>MAGMKTASGDYIDSSWELRVFVGEEDPEAESVTLRVTGESHIGGVLLKIVEQINRKQDWSDHAIWWEQKRQWLLQTHWTLDKYGILADARLFFGPQHRPVILRLPNRRALRLRASFSQPLFQAVAAICRLLSIRHPEELSLLRAPEKKEKKKKEKEPEEELYDLSYHMLSRPQPPPDPLLLQRLPRPSSLSDKTQLHSRWLDSSRCLMQQGIKAGDALWLRFKYYSFFDLDPKTDPVRLTQLYEQARWDLLLEEIDCTEEEMMVFAALQYHINKLSQSGEVGEPAEGLNPYGLVAPRFQRKFKAKQLTPRILEAHQNVAQLSLAEAQLRFIQAWQSLPDFGISYVMVRFKGSRKDEILGIANNRLIRIDLAVGDVVKTWRFSNMR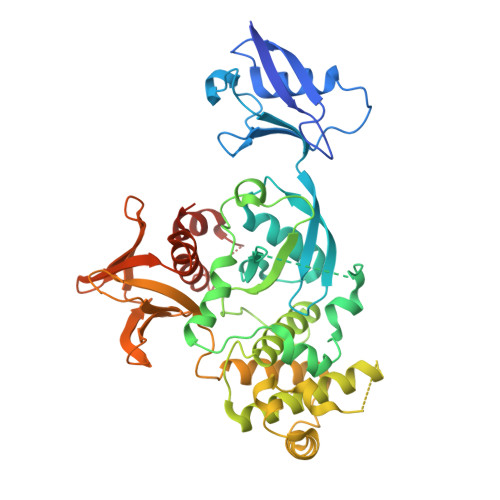QWNVNWDIRQVAIEFDEHINVAFSCVSASCRIVHEYIGGYIFLSTRERARGEELDEDLFLQLTGGHEAFLEHHHHHH[2x]>ILVRKNIHSLSHHEAEELRDALYKLQNDESHGGYEHIAGFHGYPNLCPEKGDEKYPCCVHGMSIFPHWHRLHTIQFERALKKHGSHLGIPYWDWTQTISSLPTFFADSGNNNPFFKYHIRSINQDTVRDVNEAIFQQTKFGEFSSIFYLALQALEEDNYCDFEVQYEILHNEVHALIGGAEKYSMSTLEYSAFDPYFMIHHASLDKIWIIWQELQKRRVKPAHAGSCAGDIMHVPLHPFNYESVNNDDFTRENSLPNAVVDSHRFNYKYDNLNLHGHNI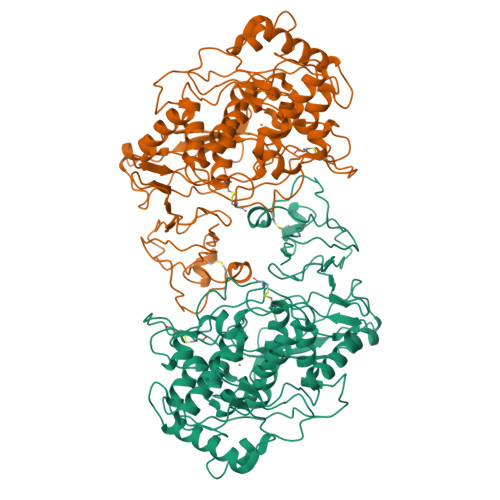EELEEVLRSLRLKSRVFAGFVLSGIRTTAVVKVYIKSGTDSDDEYAGSFVILGGAKEMPWAYERLYRFDITETVHNLNLTDDHVKFRFDLKKYDHTELDASVLPAPIIVRRPNNAVFDIIEIPIGKDVNLPPKVVVKRGTKIMFMSVDEAVTTPMLNLGSYTAMFKCKVPPFSFHAFELGKMYSVESGDYFMTASTTELCNDNNLRIHVHVD[2x]> AGPWADIMQG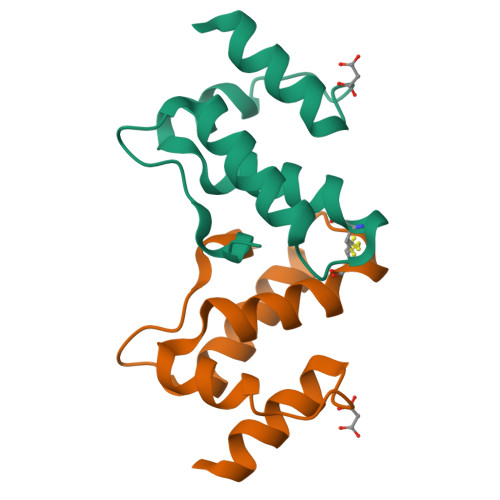PSESFVDFANRLIKAVEGSDLPPSCRAPVIIDCFRQKSQPDIQQLIRTAPSTLTTPGEIIKYVLDRQ> GSMTSGT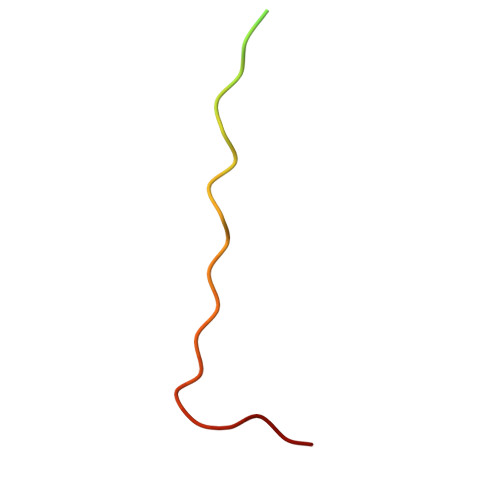SGTSGGPSPPPTWPHLQLCYLQPPPV>[2x]SNEFTYSYLFRMISHEMKQKADQKLEQFDITNEQGHTLGYLYAHQQ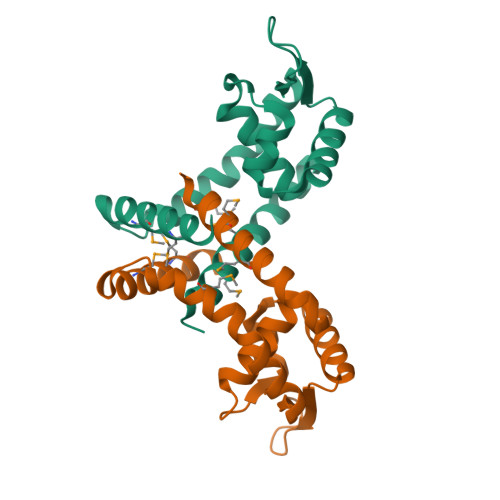DGLTQNDIAKALQRTGPTVSNLLRNLERKKLIYRYVDAQDTRRKNIGLTTSGIKLVEAFTSIFDEMEQTLVSQLSEEENEQMKANLTKMLSSLQ>[2x]RSPWNRIPESGGDNSVFDIFELTGAARKGSGRRLVKGPDPSSPAFRIEDANLIPPVPDDKFQDLVDAVR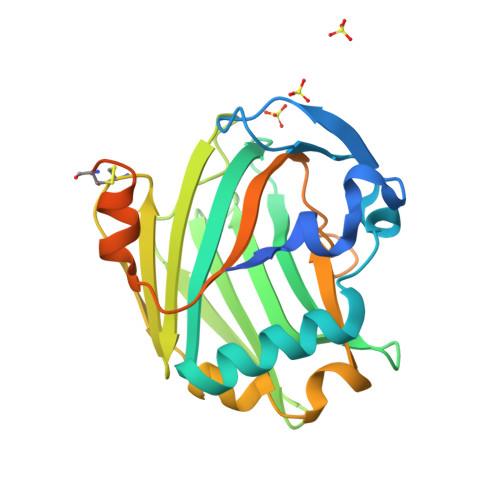TEKGFLLLASLRQMKKTRGTLLALERKDHSGQVFSVVSNGKAGTLDLSLTVQGKQHVVSVEEALLATGQWKSITLFVQEDRAQLYIDCEKMENAELDVPIQSVFTRDLASIARLRIAKGGVNDNFQGVLQNVRFVFGTTPEDILRNKGCSSSTSVLLTLDNNVVNGSSPAIRTNTGHHHHHH4-chloro-N-(4-chlorobenzyl)-5-nitro-1H-pyrazole-3-carboxamide | C11 H8 Cl2 N4 O3 | 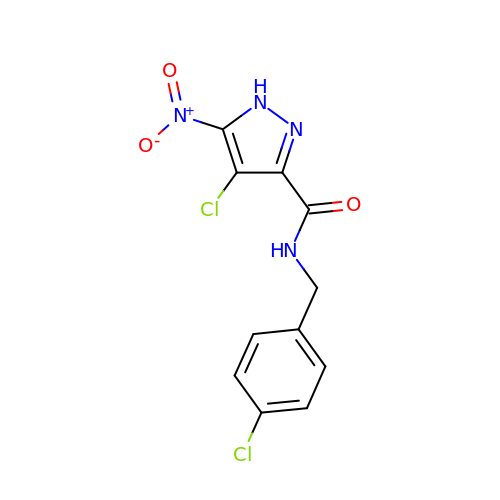APWLSOMMVQHYQM-UHFFFAOYSA-N> GSRTDLLNVCMDAKHHKTKPGPEDKLHDQCSPWKKNACCTASTSQELHKDTSRLYNFNWDHCGKMEPACKRHFIQDTCLYECSPNLGPWIQQVNQSWRKERFLDVPLCKEDCQRWWEDCHTSHTCKSNWHRGWDWTSGV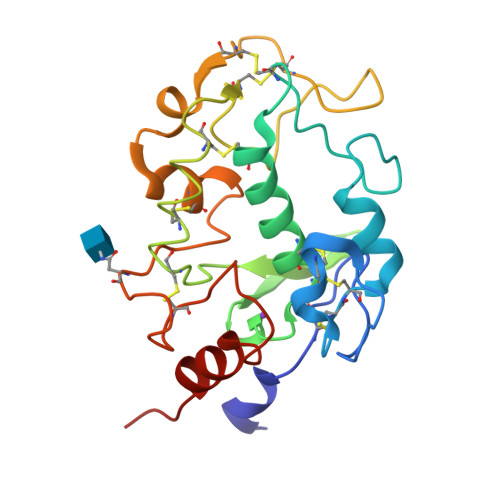NKCPAGALCRTFESYFPTPAALCEGLWSHSYKVSNYSRGSGRCIQMWFDSAQGNPNEEVARFYAAAMH>[2x]GPLGSPEFSKRSSDPSPAGDNEIERVFVWDLDETIIIFHSLLTGTFASRYGKDTTTSVRIGLMMEEMIFNLADTHLFFNDLEDCDQIHVDDVSSDDNGQDLSTYNFSADGFHSSAPGANLCLGSGVHGGVDWMRKLAFRYRRVKEMYNTYKNNVGGLIGTPKRETWLQLRAELEALTDLWLTHSLKALNLINSRPNCVNVLVTTTQLIPALAKVLLYGLGSVFP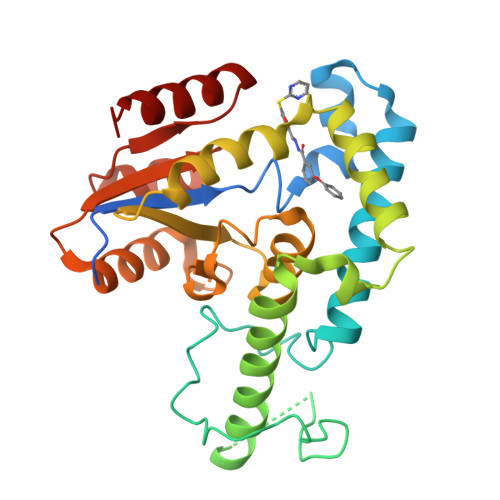IENIYSATKTGKESCFERIMQRFGRKAVYVVIGDGVEEEQGAKKHNMPFWRISCHADLEALRHALELEYL> MSDIRHSLLRRDALSAAKEVLYHL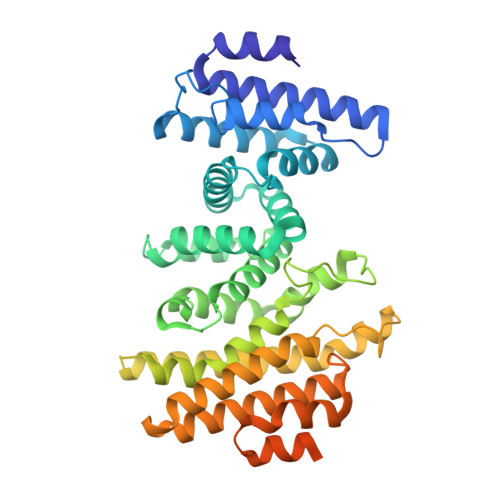DIYFSSQLQSAPLPIVDKGPVELLEEFVFQVPKERSAQPKRLNSLQELQLLEIMCNYFQEQTKDSVRQIIFSSLFSPQGNKADDSRMSLLGKLVSMAVAVCRIPVLECAASWLQRTPVVYCVRLAKALVDDYCCLVPGSIQTLKQIFSASPRFCCQFITSVTALYDLSSDDLIPPMDLLEMIVTWIFEDPRLILITFLNTPIAANLPIGFLELTPLVGLIRWCVKAPLAYKRKKKPPLSNGHVSNKVTKDPGVGMDRDSHLLYSKLHLSVLQVLMTLQLHLTEKNLYGRLGLILFDHMVPLVEEINRLADELNPLNASQEIELSLDRLAQALQVAMASGALLCTRDDLRTLCSRLPHNNLLQLVISGPVQQSPHAALPPGFYPHIHTPPLGYGAVPAHPAAHPALPTHPGHTFISGVTFPFRPIR>GPGSMAAWSGNPSFELFQLPEEHIALREAIRALAEKEIAPYAAEVDEKARFPEEALAALNSSGFSAIHVPEEYGGQGADSVATCIVIEEVARVDCSASLIPAVNKLGTMGLILRGSEELKKQVLPAVASGEAMASYALSEREAGSDAASMRTRAVADGDDWILNGSKCWITNGGKSTWYTVMAVTDPDKGANGISAFMVHKDDEGFTVGPKERKLGIKGSPTTELYFENCRIPGDRIIGEPGTGFKTALATLDHTRPTIGAQAVGIAQGALDAAIAYTKERKQF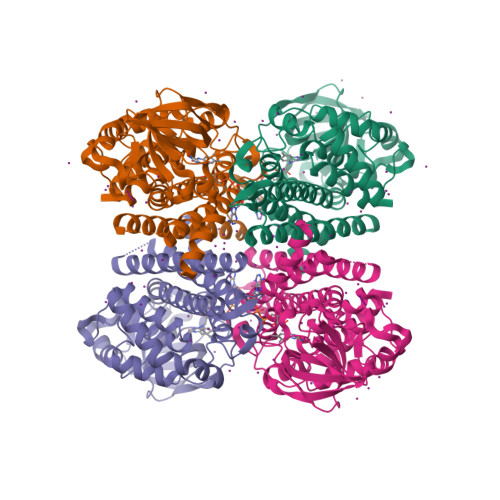GRPVSDNQGVQFMLADMAMKIEAARLMVYSAAARAERGEGDLGFISAASKCFASDVAMEVTTDAVQLFGGYGYTQDFPVERMMRDAKITQIYEGTNQIQRVVMSRALLR[4x]>MGCWGRNRGRLLCMLALTFMFMVLEVVVSRVTSSLAMLSDSFHMLS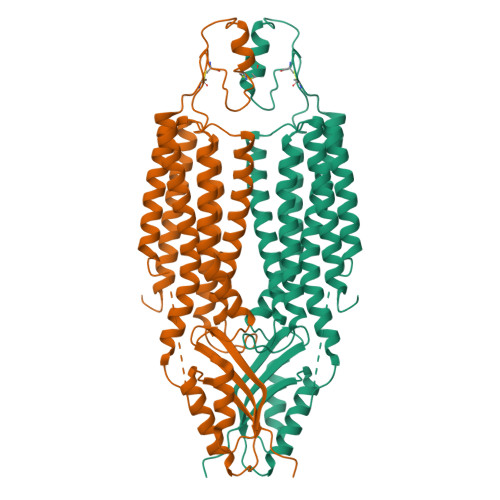DVLALVVALVAERFARRTHATQKNTFGWIRAEVMGALVNAIFLTGLCFAILLEAIERFIEPHEMQQPLVVLGVGVAGLLVNVLGLCLFHHHSGFSQDSGHGHSHGGHGHGHGLPKGPRVKSTRPGSSDINVAPGEQGPDQEETNTLVANTSNSNGLKLDPADPENPRSGDTVEVQVNGNLVREPDHMELEEDRAGQLNMRGVFLHVLGDALGSVIVVVNALVFYFSWKGCSEGDFCVNPCFPDPCKAFVEIINSTHASVYEAGPCWVLYLDPTLCVVMVCILLYTTYPLLKESALILLQTVPKQIDIRNLIKELRNVEGVEEVHELHVWQLAGSRIIATAHIKCEDPTSYMEVAKTIKDVFHNHGIHATTIQPEFASVGSKSSVVPCELACRTQCALKQCCGTLPQAPSGKDAEKTPAVSISCLELSNNLEKKPRRTKAENIPAVVIEIKNMPNKQPESSL[2x]> RDPGPRRSESPPGPGGDASLLARLFEHPLYRVAVPPLTEEDVLFNVNSDTRLSPKAAENPDWPHAGAEGAEFLSPGEAAVDSYPNWLKFHIGINRYELYSRHNPAIEALLHDLSSQRITSVAMKSGGTQLKLIMTFQNY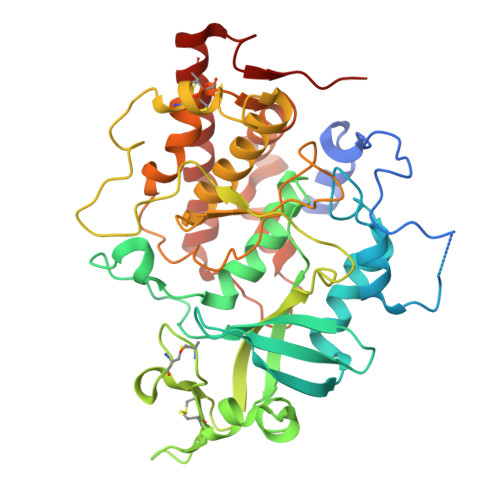GQALFKPMKQTREQETPPDFFYFSDYERHNAEIAAFHLDRILDFRRVPPVAGRMVNMTKEIRDVTRDKKLWRTFFISPANNICFYGECSYYCSTEHALCGKPDQIEGSLAAFLPDLSLAKRKTWRNPWRRSYHKRKKAEWEVDPDYCEEVKQTPPYDSSHRILDVMDMTIFDFLMGNMDRHHYETFEKFGNETFIIHLDNGRGFGKYSHDELSILVPLQQCCRIRKSTYLRLQLLAKEEYKLSLLMAESLRGDQVAPVLYQPHLEALDRRLRVVLKAVRDCVERNGLHSVVDDDLDTEH The l,d-transpeptidase LdtMt2, which is responsible for the formation of 3 → 3 cross-links in the cell wall peptidoglycan, has been identified as essential for M. tuberculosis virulence. The extramembrane section of LdtMt2 consists of three domains, two of which have an immunoglobulin-related fold, and the catalytic domain which has an ErfK/YbiS/YhnG fold. The LdtMt2 active site within the catalytic domain is bordered by a flexible loop (residues 300–323), sometimes referred to as the active site “lid”, which creates two entrances to the active site: the inner and outer cavities. The Ldt mechanism is proposed to be analogous to that proposed for the PBPs, although employing a catalytic triad analogous to that observed in some cysteine-proteases, involving Cys354, His336 and Ser337, for the formation of the cross-link between the donor and acceptor stem substrates.

A crystal structure of LdtMt2 reacted with cyanamide 31 manifested covalent modification of Cys354 with formation of a carbamoyl group, likely resulting from initial formation of cyanated cysteine followed by hydrolysis. The carbamoyl group was directed towards the oxyanion hole (the respective distances of the carbonyl oxygen to the backbone nitrogens of His352, Gly353 and Cys354: 3.6 Å, 3.5 Å and 3.1 Å). Further polar interactions were observed between the nitrogen of the carbamoyl group and the sidechain of Tyr318 (3.4 Å in chain A) and the backbone carbonyl of Gly332 (3.4 Å in chain A). In certain cases, this was accompanied by an additional modification of +17 Da, which likely reflects the addition of water to the transferred nitrile group to give an S-carbamoyl cysteine residue. Interestingly, in some cases we observed hydrolysis of the S-nitrile group to give an S-carbamoyl group, as validated by crystallography in the case of 31. Of the LdtMt2 inhibitor classes identified here, the cyanamides 22–36 are of particular mechanistic interest, as they are electrophilic agents that cyanate Cys354 with high inhibitory potency.

>[2x]QSDLLVPKLTASVTDGAVGVTVDAPVSVTAADGVLAAVTMVNDNGRPVAGRLSPDGLRWSTTEQLGYNRRYTLNATALGLGGAATRQLTFQTSSPAHLTMPYVMPGDGEVVGVGEPVAIRFDENIADRGAAEKAIKITTNPPVEGAFYWLNNREVRWRPEHFWKPGTAVDVAVNTYGVDLGEGMFGEDNVQTHFTIGDEVIATADDNTKILTVRVNGEVVKSMPTSMGKDSTPTANGIYIVGSRYKHIIMDSSTYGVPVNSPNGYRTDVDWATQISYSGVFVHSAPWSVGAQGHTNTSHGCLNVSPSNAQWFYDHVKRGDIVEVVNTVGGTLPGIDGLGDWNIPWDQWRAGNAKA>SQLTTESMPFNVAEGKEVLLLVHNLPQQLFGYSWYKGERVDGNRQIVGYAIGTQQATPGPANSGRETIYPNASLLIQNVTQNDTGFYTLQVIKSDLVNEEATGQFHVY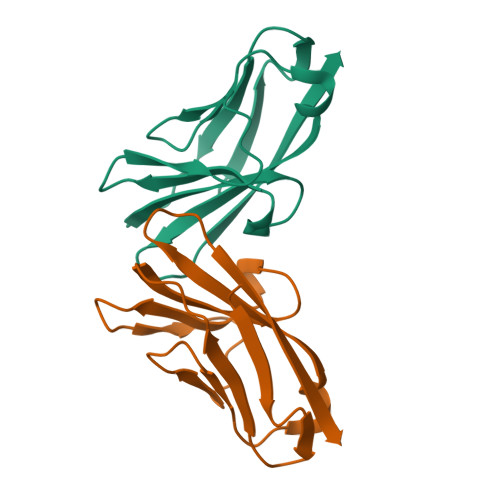[4x]> GAGCAGACCCG;> ACGGCACTCA;> CGCGT;> TCTGAGTGCGGTCTGC

In this work, we exhaustively probe the ability of all 36 immobile HJ sequences to form DNA crystals in two different designed systems. Three separate self-assembling DNA crystal systems are described in this report: the “4 × 5” and “4 × 6” designs (collectively referred to as the 4 × N systems), and a third construct with a “scrambled” sequence variant of the 4 × 6 lattices. Self-assembly was mediated by three constituent oligonucleotides: (S1) containing four sequence repeats of either 5 or 6 bases; (S2) composed of 21 bases containing complementary regions to both (S1); and (S3) which forms the second junction crossover. The HJ serves as the fundamental component at the core of each unit, and the ultimate assembly of the full lattice is facilitated by the complementary 2-base sticky ends that tail each duplex.

The aperiodic lattice contained cavities with widths of 1.0 and 1.7 nm at alternating intervals, and yielded exceedingly small pore volumes of ~24 nm3. The cavity volumes of the P3221 lattices were calculated based upon the 3-nm edges of the pores along the three-fold symmetry axis of the crystal with a triangular prism height of 6.1 nm, corresponding to the average c-axis of the unit cell. However, in the majority of the crystal structures reported here, the cacodylate anion indeed fits best into the electron density map of our X-ray structures, due to the presence of sodium cacodylate in the crystallization solution.> GSHMLSDEQMQIINSLVEAHHKTYDDSYSDFVRFRPPVREGPVTRSASRAASLHSLSDASSDSFNHSPESVDTKLNFSNLLMMYQDSGSPDSSEEDQQSRLSMLPHLADLVSYSIQKVIGFAKMIPGFRDLTAEDQIALLKSSAIEIIMLRSNQSFSLEDMSWSCGGPDFKYCINDVTKAGHTLELLEPLVKFQVGLKKLKL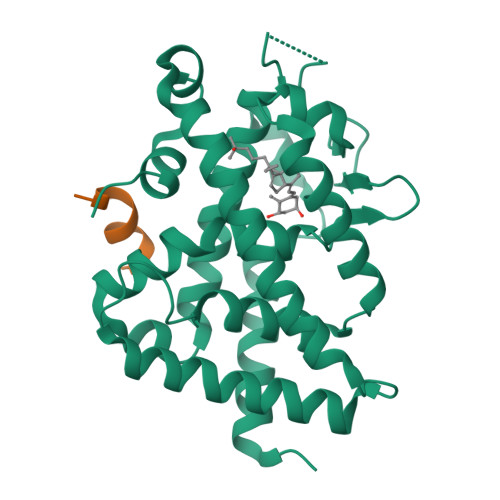HEEEHVLLMAICLLSPDRPGVQDHVRIEALQDRLCDVLQAYIRIQHPGGRLLYAKMIQKLADLRSLNEEHSKQYRSLSFQPEHSMQLTPLVLEVFGSEVS;> RHKILHRLLQEGSPS>[2x]QINQVRPKLPLLKILHAAGAQGEMFTVKEVMHYLGQYIM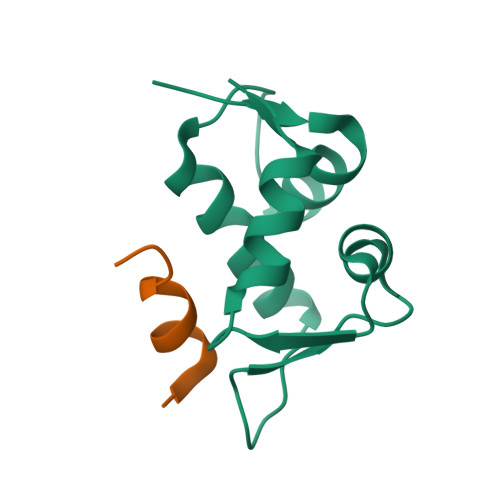VKQLYDQQEQHMVYCGGDLLGELLGRQSFSVKDPSPLYDMLRKNLVTLAT;>[2x]ETFEHWWSQLLS>LGLSITGLGVQYPPYSLGPDAIDILSKRYHPESPAMKKVLAINRYTGIDQRSSIGNPDHPLVNKPNPPTVKELHEVFMSDGVPLAVEASRKAMAEARLVPAQITHMVSTTCTDSANPGYDHYVAKELGLSDRLEKVLLHGIGCS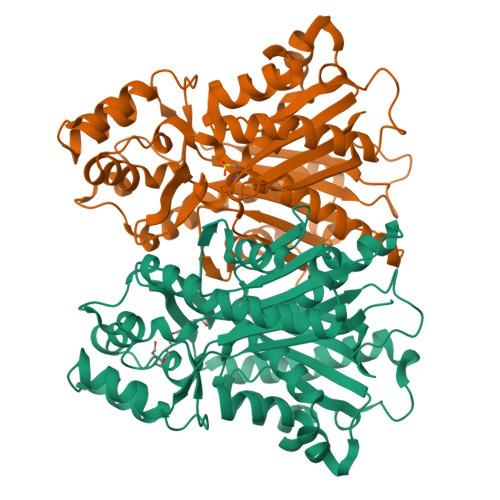GGLAALRTAANLCLGHTARGKPARILVLALEVSTTMVRSELESIDALQETRIGIALFSDCASAVILSNGIGEAPGKPAIYDLLGWENRVIPDSEHDLGGDVDPMGWKVVLSPRVPVLAKASLQPTYADLLSSLQDQLPSSYQKPADFDWAMHPGGATILSGAESAMGLTPEHMRASYDRYINHGNSSSATIFSVLNRLREKDMDALAPGGKVKEYVVGCAFGPGINVEMCMLKRR[4x]>MARDHRKIGKQLDLYHMQEEAPGMVFWHNDGWTIFRELEVFVRSKLKEYQYQEVKGPFMMDRVLWEKTGHWDNYKDAMFTTSSENREYCIKPMNCPGHVQIFNQGLKSYRDLPLRMAEFGSCHRNEPSGSLHGLMRVRGFTQDDAHIFCTEEQIRDEVNGCIRLVYDMYSTFGFEKIVVKLSTRPEKRIGSDEMWDRAEADLAVALEENNIPFEYQLGEGAFYGPKIEFTLYDCLDRAWQCGTVQLDFSLPSRLSASYVGEDNERKVPVMIHRAILGSMERFIGILTEEFAGFFP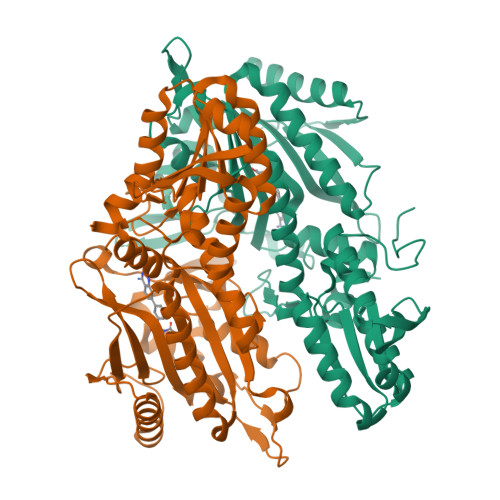TWLAPVQVVIMNITDSQSEYVNELTQKLSNAGIRVKADLRNEKIGFKIREHTLRRVPYMLVCGDKEVESGKVAVRTRRGKDLGSMDVNEVIEKLQQEIRSRSLKQLEELEHHHHHH[2x]> ATVQSPDGNIKIIISDEQSTPSYSISFKNKTVINNSALGFEFKQHAPFSNSFKITKV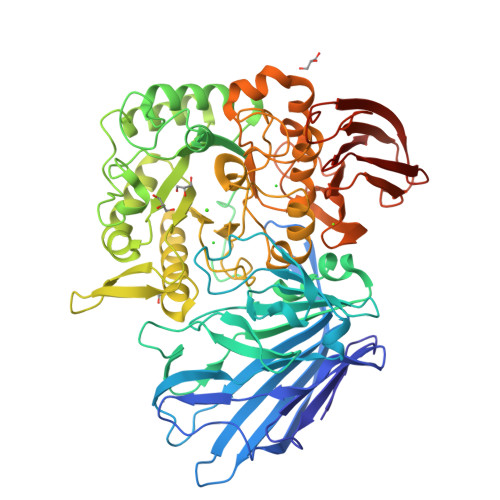QQQSTNTQWQQPWGERQTVVDQHNEVTVTFAKPQPQGGTYSVRFKAFDSGVGFRYEVPKQAGLNNIEITKELTEFAVNNSHTATAWWIPARGWNRYEYVYNTTPLNDAALVHTPFTFKNQDGVHISIHEAALVDYAAMVLNQRRPGVFQADLTPWSSGVAVKKQGAFNTPWRTIQIGEKAVDLVNSDIILNLNEPNKLGDVSWVKPGKYIGIWWGMHINTHTWGSGDKHGATTKNTKYYMDFAAKYGFDGVLVEGWNTGWDGDWFFNGDVFSFTQPYDDFDIAALTKYSKQTGVQLIGHHETSGNVSNYRKQMADAFALYEKSNVSQVKTGYVADGGNIKRIDKNGIARHEWHDGQFMVNEYLHNVKLAAKHKISINTHEPIKDTGLRRTYPNWITREGARGQEFNAWGTPPNPPEHISMLAFTRMLAGPMDFTPGIFDLSFNGLGANTNRPQTTLAKQLALYVVLYSPIQMAADLPKNYLAKPDAFQFIQDVPTDWQQSIALDGAVGDFIVFARKERKRDKYTGNDWYLGAVTDEQARTIEISLDFLDNGKQFEAHIYKDGKNAEWKNNPYDLTIEKRLVTASDKLTLKLATSGGTAIRFKALLEHHHHHH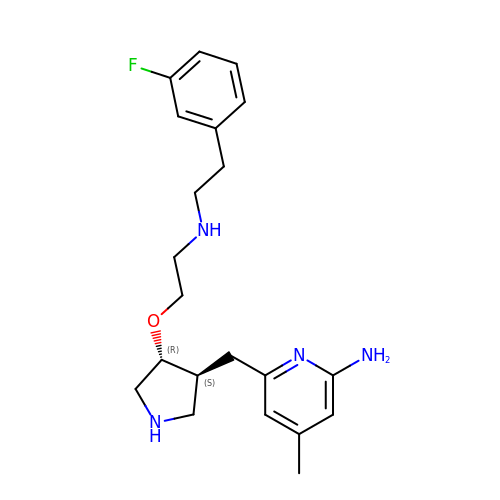6-{[(3S,4R)-4-(2-{[2-(3-fluorophenyl)ethyl]amino}ethoxy)pyrrolidin-3-yl]methyl}-4-methylpyridin-2-amine | C21 H29 F N4 O | NESZTSPBRDBHCW-PXNSSMCTSA-N>[8x]MARNIVVEEIVRTPVEMQQVELVERKGIGHPDSIADGIAEAVSRALCREYIRRYGVILHHNTDQVEVVGGRAYPRFGGGEVVKPIYILLSGRAVELVDQELFPVHEVAIKAAKNYLKNAIRHLDVENHVIID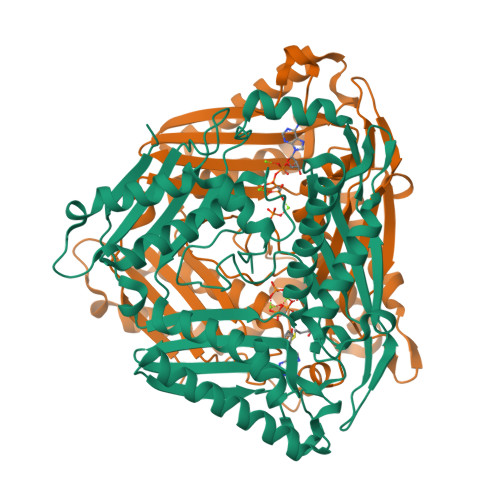SRIGQGSVDLVSVFNKARENPIPLANDTSFGVGYAPLSETERLVLETEKLLNSEKFKKEYPAVGEDIKVMGLRRGNEIDLTIAAAIVDSEVATPKEYLEVKDKIKEAVEELAKEITSRKVNIYVNTADDPERGIYYITVTGTSAEAGDDGSVGRGNRVNGLITPNRHMSMEAAAGKNPVSHVGKIYNILAMLIAEDIAKTLPVEEVYVRILSQIGKPIDQPLVASIQVIPKPGHSVKEFEKDAYSIADEWLANITKVQKMILEDKISVF> KLPTNLAYERSIDPSDVCFFVVWPDDRKTPLTYNSRTLLGQMEAKSLAYDVSGQPIKSATAEALAQGNPHQVDFCHVPYGASHIECSFSVSFSSELRQPYKCNSSKVKQTLVQLVELYETKIGWTELATRYLMNICNGKWLWKNTRKAYCWNIVLTPWPWNGEKVGFEDIRTNYTSRQDFKNNKNWSAIVEMIKTAFSSTDGLAIF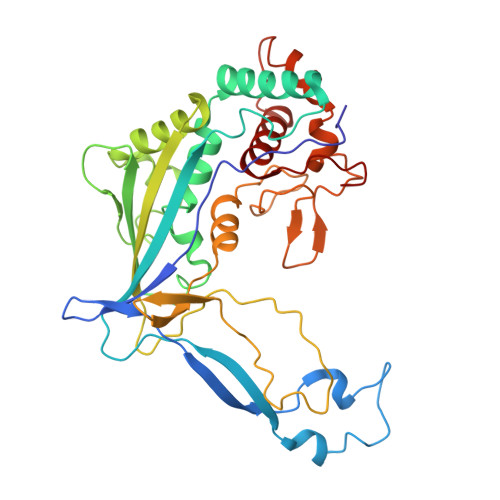EVRATLHLPTNAMVRPSQVFTEKEAAAAAAAATQNSRVFQSTTIDGERSPILGAFKTGAAIATIDDWYPEATEPLRVGRFGVHREDVTCYRHPSTGKDFFSILQQAEHYIEVLSANKTPAQETINDMHFLMANLIKGGMFQHKGD>[4x]MSNEYDEYIANHTDPVKAINWNVIPDEKDLEVWDRLTGNFWLPEKIPVSNDIQSWNKMTPQEQLATMRVFTGLT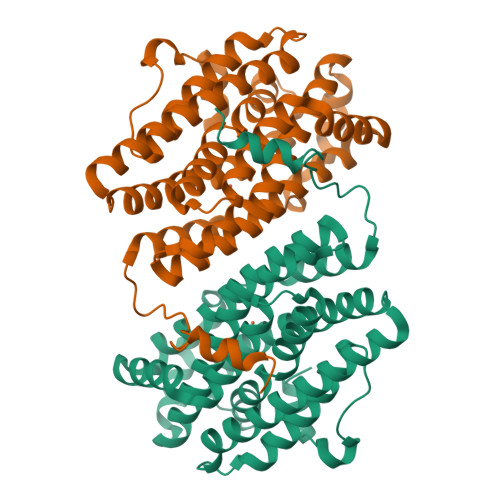LLDTIQGTVGAISLLPDAETMHEEAVYTNIAFMESVHAKSYSNIFMTLASTPQINEAFRWSEENENLQRKAKIIMSYYNGDDPLKKKVASTLLESFLFYSGFYLPMYLSSRAKLTNTADIIRLIIRDESVHGYYIGYKYQQGVKKLSEAEQEEYKAYTFDLMYDLYENEIEYTEDIYDDLGWTEDVKRFLRYNANKALNNLGYEGLFPTDETKVSPAILSSLSPNADENHDFFSGSGSSYVIGKAEDTTDDDWDF>[2x]MDRMKIEAVIFDWAGTTVDYGCFAPLEVFMEIFHKRGVAITAEEARKPMGLLKIDHVRALTEMPRIASEWNRVFRQLPTEADIQEMYEEFEEILFAILPRYASPINGVKEVIASLRERGIKIGSTTGYTREMMDIVAKEAALQGYKPDFLVTPDDVPAGRPYPWMCYKNAMELGVYPMNHMIKVGDTVSDMKEGRNAGMWTVGVILGSSELGL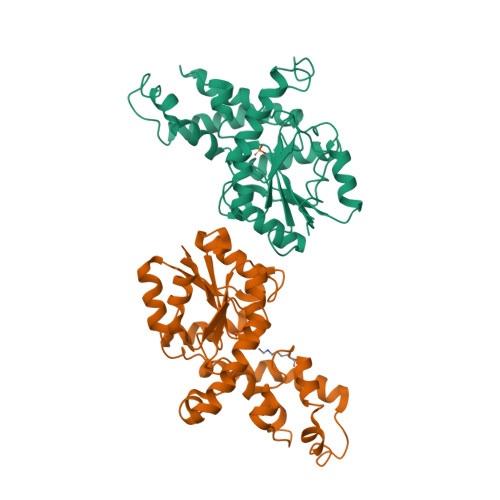TEEEVENMDSVELREKIEVVRNRFVENGAHFTIETMQELESVMEHIEKQELIIS Type IV pili (T4P) represent one of the most common varieties of surface appendages in archaea. These filaments, assembled from small pilin proteins, can be many microns long and serve diverse functions, including adhesion, biofilm formation, motility, and intercellular communication. In this study, we present the high-resolution cryo-EM structures of the Saccharolobus islandicus REY15A mono-pilus and tri-pilus and demonstrate that archaeal type IV pilins can also polymerize into dramatically different filament structures.

The cells grown in rich medium (MTSVY), produced a single variety of T4P which were very similar to the adhesive Aap pili previously reported for S. islandicus LAL14/16, with a slightly improved resolution (3.9 Å versus 4.1 Å). We denote this type of T4P as mono-pilus (see below). The mono-pilus has an asymmetrical unit containing a single pilin with a helical rise of ~4.95 Å and a helical rotation of ~104.8°, displaying a slightly right-handed 7-start feature, similar to the Aap pilus of S. islandicus LAL14/1. The REY15A mono-pilus structure adopts the known archaeal T4P two-domain fold, featuring a long N-terminal α-helix and a C-terminal globular Ig-like β-strand-rich domain. In the mono-pilus, the inner helix of a mono-pilin S0 interacts with outer domains from pilins S+4, S+7, and S+11, resulting in a total buried surface of approximately 873 Å2. In the mono-pilus, the outer domains are densely packed. The outer domain of S0 interacts with six other outer domains, exhibiting an extensive total buried surface area of 1,574 Å2. Three out of those six interfaces are unique (with the other three related by symmetry), with buried surface area ranging from 236 to 300 Å2. Previous work has demonstrated that a closely related mono-pilus exhibits remarkable stability under extremely harsh conditions, such as boiling in GuCl or pepsin digestion. This can be attributed to the fact that the inner hydrophobic helices of the mono-pilus are completely encased by the outer domains, which are further armored by heavy glycosylation. Under conditions of nutrient limitation, S. islandicus REY15A cells predominantly express tri-pili, although mono-pili and flagella are also present at low levels; however, in the rich medium, the cells exclusively express the mono-pilus.

> MNMISRRKNAKALSGAVTALILVIASVIIALVVVGFAFGLFGAFTGQGTVTQVGTATLSAGTGTLTVTLKNTGAATQVTGAIINGNAASVSGQVTISAGQNTYSISLGGISSSTLQNLVGSTISLTLQLSNGQTVTVSAIITS N-[(1S)-5-amino-1-(chloroacetyl)pentyl]-4-methylbenzenesulfonamide | C14 H21 Cl 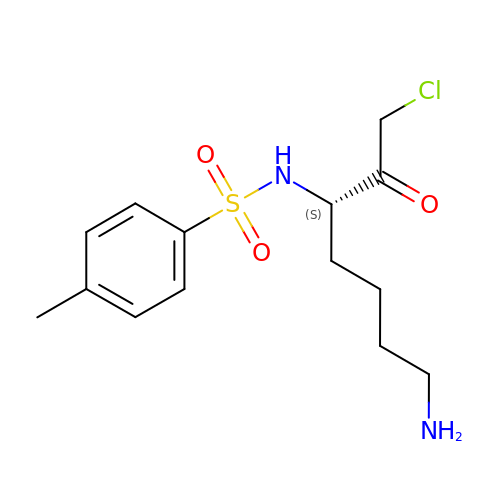N2 O3 S | RDFCSSHDJSZMTQ-ZDUSSCGKSA-N D-galactaric acid | C6 H10 O8 | 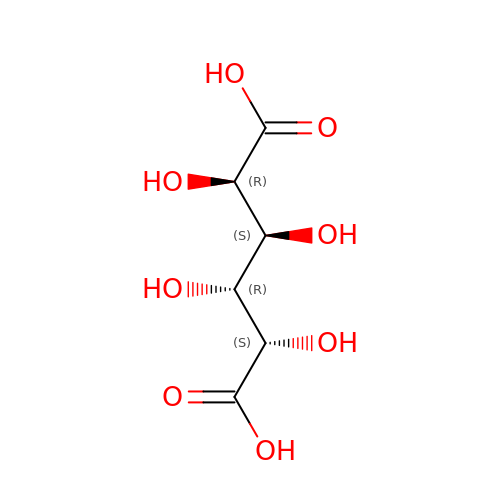DSLZVSRJTYRBFB-DUHBMQHGSA-N>[2x]MPNPPAKEDTWAFGPIGSPFP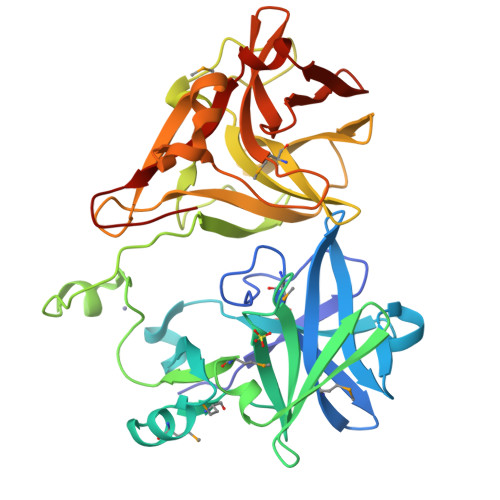DNPVKALGQQNMYVALWYKNGRPMHGRAWNNGGVIECSFPYNKSELTGVKDLGGQIQVLQYKGNHLSLGYWYNWIKYSDRFDKMDKGAEMLRCGDSFPILWSERPGGALLGYADNKTEIARFSHDGKVDEVSGSALANMLIIARELKGGPPYCECEECKSEPPKPIVRVTLNEWADFRCGDPWPTVGTPVRALGRSLDTLPGENPDQYVALWYQSGEPVMGRIWNDGGKIAACFGWGGHEYRQKIGSIQILYELPEAIRGFDYDWKPFPEAAQFGAKEWIPVHVDHHKGNISPAVLIVDGKEILGKADIRNERATIGYGGTEKVLVGPAVHSCMVLCRKAKPGCTID>[3x]MRRLNRKNNEALKKLNDRQRKVLYCIVREYIENKKPVSSQRVLEVSNIEFSSATIRNDMKKLEYL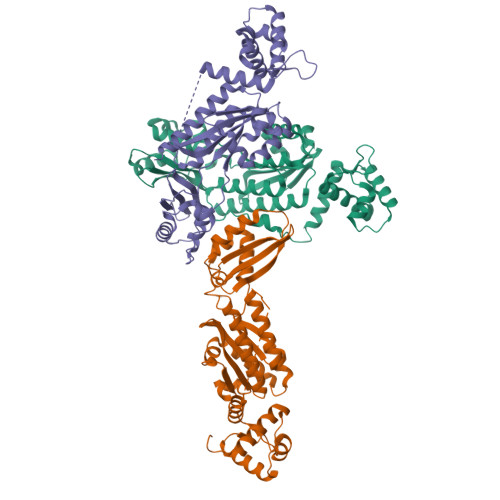GYIYQPHTSAGRIPTDKGLRFYYEEMLKISKETSEADLAVETFKSMPLADPEKVLFLAGNLLARLTEGYVLIERPNTRDLKILRVMLIPVSEDYLIFSILTEFGVSKVTPIKTQERLNWEEIERQLNFLLRGRTVGEVLMGKIESLKGSGFLRLIESLIGETVERYLDAGLENLLKDETLTLEDIRNLLEEVKDQKFLESLVGEGITVRIGREIGRKKLEKFAVFSGKYFKGESPIGSVYLFTSKVTKYDRNHRVFEYILNRLSEYFTSTSRR2-deoxy-6-O-phosphono-alpha-D-glucopyranose 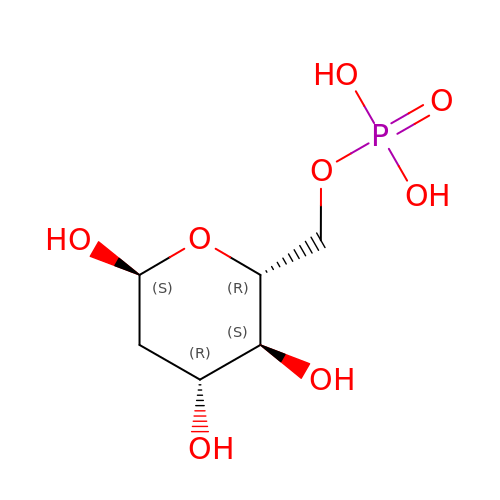| C6 H13 O8 P | UQJFZAAGZAYVKZ-ZXXMMSQZSA-N>MASHHHHHHDYDGATTENLYFQGSMDVVDPDIFNRDPRDHYDLLQRL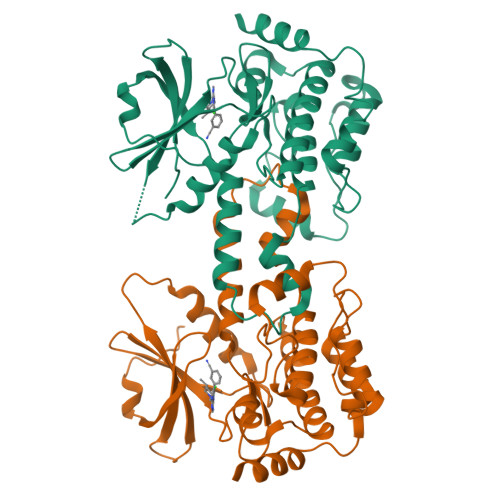GGGTYGEVFKARDKVSGDLVALKMVKMEPDDDVSTLQKEILILKTCRHANIVAYHGSYLWLQKLWICMEFCGAGSLQDIYQVTGSLSELQISYVCREVLQGLAYLHSQKKIHRDIKGANILINDAGEVRLADFGISAQIGAELARRLEFIGTPYWMAPEVAAVALKGGYNELCDIWSLGITAIELAELQPPLFDVHPLRVLFLMTKSGYQPPRLKEKGKWSAAFHNFIKVTLTKSPKKRPSATKMLSHQLVSQPGLNRGLILDLLDKLKNPGKGPSIGDIEDEE[6x]N~4~-(2-chlorophenyl)-N~2~-[4-(1H-tetrazol-5-yl)phenyl]pyrimidine-2,4-diamine 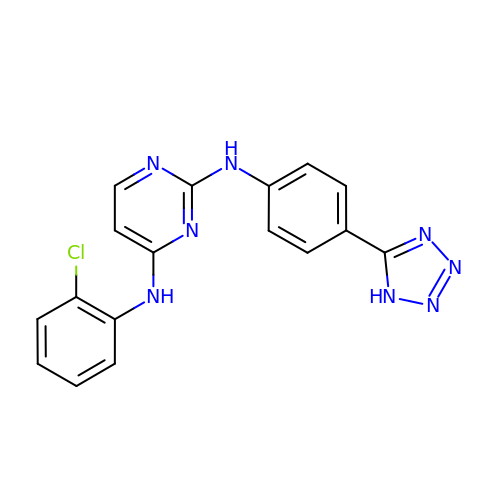| C17 H13 Cl N8 | GADYBZMYJCZJLX-UHFFFAOYSA-N>[2x]SFMDRKEVVNIQTWINKPDIKHHFPCKEVKESGHMFPSHLLVTATHMYCLREILSRKGLAYIQSRQALNSVVKITSKKKHPELITFKYGNSSASGIEILAIERYLIPNAGDATRAIKQQIMK;>[2x]DDNTLYHRGFTED

The Golgi-localized golgins golgin-97 and golgin-245 capture transport vesicles arriving from endosomes via the protein TBC1D23. The amino-terminal domain of TBC1D23 binds to the golgins, and the carboxyl-terminal domain of TBC1D23 captures the vesicles, but how it recognizes specific vesicles was unclear. A search for binding partners of the carboxyl-terminal domain unexpectedly revealed direct binding to carboxypeptidase D and syntaxin-16, known cargo proteins of the captured vesicles. Binding is via a threonine-leucine-tyrosine (TLY) sequence present in both proteins next to an acidic cluster.

Peptides corresponding to the relevant regions of syntaxin-16 and CPD showed robust enthalpic-dominated binding to the C-terminal domain by isothermal titration calorimetry (ITC) with affinities of ~1.4 and 10.6 μM, respectively, and a stoichiometry of 1:1. The previously observed strand-exchanged dimer was absent with the homodimeric C-terminal tail–mediated interface being replaced by the peptide. Thus, the structure elucidates how the syntaxin-16 peptide binds to the C-terminal domain of TBC1D23. The peptide extends TBC1D23’s β sheet by adopting a twisted β augmentation mode of interaction with strand 5 and buries ~670 Å2 of the C-terminal domain’s solvent accessible surface area, a similar sized interface to those seen previously for other trafficking motif–binding proteins that have a similar KD of interaction. The Thr212 in the acidic TLY motif of syntaxin-16 packs its methyl group against the alkyl chain of Lys628 that orients the hydroxyl group toward the solvent to stabilize a somewhat strained backbone conformation. This allows the side chains of the leucine and tyrosine residues to be splayed apart and simultaneously buried into neighboring hydrophobic pockets in the domain. As a result, the acidic residues Asp209 and Asp210 of syntaxin-16 are in close proximity to three basic residues (Lys632 to Lys634) in the C-terminal domain of TBC1D23, which would allow a direct electrostatic interaction. Lys672 of TBC1D23 hydrogen bonds via its amine group to the carboxyl peptide bond of Lys213 in the TLY in syntaxin-16; mutation to alanine (K672A) weakened binding ~20 fold (KD ~ 30 μm). The structure indicates that recognition of the acidic cluster and the TLY triad are the critical factors in driving peptide binding and specificity.> GPLGSPEFMALAVAPWGRQWEEARALGRAVRMLQRLEEQCVDPRLSVSPPSLRDLLPRTAQLLREVAHSRRAAGGGGPGGPGGSGDFLLIYLANLEAKSRQVAALLPPRGRRSANDELFRAGSRLRRQLAKLAIIFSHMHAELHALFPGGKYCGHMYQLTKAPAHTFWRESCGARCVLPWAEFESLLGTCHPVEPGCTALALRTTIDLTCSGHVSIFEFDVFTRLFQPWPTLLKNWQLLAVNHPGYMAFLTYDEVQERLQACRDKPGSYIFRPSCTRLGQWAI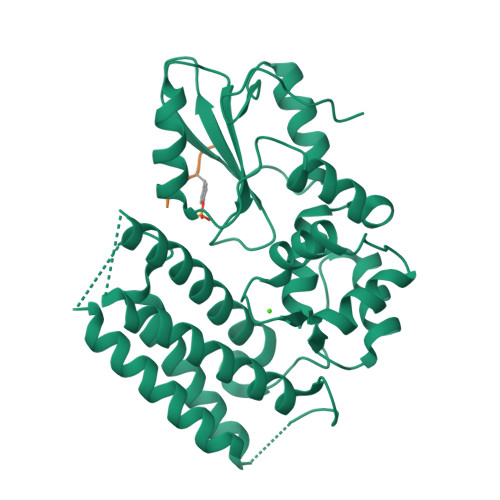GYVSSDGSILQTIPANKPLSQVLLEGQKDGFYLYPDGKTHNPDLTELG;> RLIEDNEYTARQG The type VI secretion system (T6SS) is a widespread protein export apparatus found in Gram-negative bacteria. T6SSs mediate bacterial antagonism by facilitating the injection of toxic effector proteins into competing bacterial cells in a contact-dependent manner. Here, we present the structures of the T6SS effector RhsA from Pseudomonas protegens and its cognate T6SS spike protein, VgrG1, at 3.3 Å resolution. The rhsA operon contains genes encoding its cognate VgrG spike and Eag chaperone proteins, both of which are required for the delivery of this effector into susceptible competitors.

We previously demonstrated that a fragment of RhsA lacking its N-terminal prePAAR motif and TMD (residues 74–1486), RhsAΔTMD, is stable in the absence of its EagR1 chaperone and can be purified to homogeneity as a soluble protein when over-expressed in Escherichia coli. The raw images and 2D class averages suggest that RhsAΔTMD forms a stable dimer in solution, which facilitated structure determination due to the increased size of the particles. Subsequent image processing imposing C2 symmetry resulted in a reconstruction with a resolution of 3.3 Å from 454,740 particles. The high quality of the map allowed us to build an atomic model of 75% of the protein, comprising residues 268–275, 289–302, 305–366, 371–386, 395–871, 891–1039 and 1051–1350. The 25% of remaining unresolved regions correspond to the PAAR domain (residues 75–267) and the toxin domain (residues 1351–1486), indicating that these regions likely exhibit a high degree of flexibility. The 76 antiparallel β-strands of RhsAΔTMD spiral in an anticlockwise manner resulting in a large hollow cocoon-shaped structure with outer dimensions of 86 x 65 Å. In line with functioning to self-cleave the C-terminal toxin domain, we observed that the density of the cryo-EM map stops abruptly after tryptophan 1350. The density filling the cocoon is, for the most part, not well defined and is apparent only at a much lower density threshold compared to the rest of the map, Nevertheless, we could build three β-strands of this domain, comprising residues 1408–1413, 1420–1423 and 1458–1461, respectively, all of which interact with the inner surface of the cocoon structure. Interestingly, the density inside the Rhs cocoon not only ends after tryptophan 1350 but also before proline 305, suggesting that RhsA is proteolytically cleaved at this position as well. Our structural data show that the C-terminal aspartyl protease domain of RhsA seals the cocoon-shaped structure at one end, while the other end is capped by an N-terminal domain that adopts a smaller structure. This N-terminal domain of the barrel, formed by residues 268–386, caps the cocoon structure in a manner that is reminiscent of how a cork is used to plug a champagne bottle and thus we refer to it as the N-terminal plug domain (RhsAplug).

>[2x]MGSSHHHHHHSQDPSKTGADKGLSNLCEGIANALFPPSIQATIASGSKKVLTNNKPAARAAGIAPPTQISGDGAEEGEATDTPSATPEEGPGFLDMAKEFFSQMWRPTVASPAPGSQTKELDLVTCTKHPPMPVQYLAEGSEKVSIDGQPAVRSGDRSTCDAKVVSAGPISPNVTIGGGSVVVREIRSGKTPGVGLAVTVLMMLKGGKGKFLSNLPCMLMAGVNSFVVSQATNALTQAVVASTHPVHAATGAKVLGADDDLDFTLPGLMPIEWQRFYNSRDERRDGLLGAGWSLPYEISVQIEPHPEGGERLLYIDEQGRRIDMGSIALGAGAFSPGEGLSVRRNENGQLLIESSDGIYRLFEPLPGDSSRLRLSLLGDRNDNRLHLEYDSSGRLWLLRDTFEQAQLELSYSTLWPGRIAQVERLYPDQQREVLVSYDYDAAGDLAQVRDSEGQVQRRFAYDAGHRMIEHQLATGLRCFYQWTQFADQQWRVTRHWTDEGDSYQYDYDLEAGITQVTDSLQRLSRRRWNSQLQIVEYTDNLNQTWAFEWNDERQLLSATDPLGGRYAYSYDETGNLIAETDPLGHSHSTLWLEHWSLPQTLTDPAGESWHLRYDPRGNCIAEVDPLGQVTQYRHDAHGQVVEIIDAAGRSRKMRWNSSGQLLEHLDCSGYPTRFEYDRRGNVKAIIDALGEHTRFHYDCQGRLLSSQLADGRAEHFQRSSNGQLQGYTDPSGYTTLYQYNRRGQIRQRIDAHGRQVRFDYDAYGRLLALTNENGESYRFAWDAGNRLSEQQDLDGSAKRYGYDLLNNVVELQSHPAPYGTGLSAVPAQPIAPIIHRFERDAVGRLLAKITDDGRSQYTYDPLNQLTAASFTDNLGNQQALSFSYDALGQLLEEHTVAGSLIHRYDELGNLTQTQLPDKRWLNRLYYGSGHLHQINLDGQVVSDFQRDRLHREVLRTQGQISTRSEYDRCGRLRARLQHSSLLANTLPTAPERHLEYDDSDNLVGLAERHATGQHRQLFHYDATGRIIASQDGLQGQKETFAYDAAANLLDGPKAGAGLVVHNKLLTYQDKRYRYDAFGRMIEKRSGRRGVQRFAYDAEHRLIEVRNQTSSGETLVRMRYDVLGRRISKSEYDSQGNLLGETRFVWDGLRLLQEQRNQQTSLYVYEDLGHAPLARVDGLGAQQKIRYYHNDLNGLPQQLCEPDGHSVWQARYQVWGNTVEEIREPYYIEEQNLRFQGQYLDRETGLHFNTFRFYDPDIGRFTTPDPIGLAGGLNLYQYAPNPIGWIDPLGWICKSAYSGRRGTTKAKADLERNGFTVVGEELTMKVKHPVTQKSYRIRADIIAKDKAGNYHVFEVKNGSGKLTKNQQGSGMFDMSNPANTNGGLGGGLIKPSGATQGQFEVATKTARGTQFGGNGAQHSATFWLLRY> VISYDNYVTILDEETLKAWIAKLEKAPVFAFDTETDSLDNISANLVGLSFAIEPGVAAYIPVAHDYLDAPDQISRERALELLKPLLEDEKALKVGQNLKYDRGILANYGIELRGIAFDTMLESYILNSVAGRHDMDSLAERWLKHKTITFEEIAGKGKNQLTFNQIALEEAGRYAAEDADVTLQLHLKMWPDLQKHKGPLNVFENIEMPLVPVLSRIERNGVKIDPKVLHNHSEELTLRLAELEKKAHEIAGEEFNLSSTKQLQTILFEKQGIKPLKKTPGGAPSTSEEVLEELALDYPLPKVILEYRGLAKLKSTYTDKLPLMINPKTGRVHTSYHQAVTATGRLSSTDPNLQNIPVRNEEGRRIRQAFIAPEDYVIVSADYSQIELRIMAHLSRDKGLLTAFAEGKDIHRATAAEVFGLPLETVTSEQRRSAKAI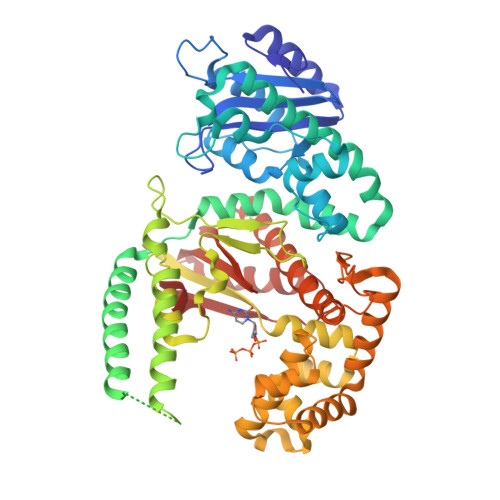NFGLIYGMSAFGLARQLNIPRKEAQKYMDLYFERYPGVLEYMERTRAQAKEQGYVETLDGRRLYLPDIKSSNGARRAAAERAAINAPMQGTAADIIKRAMIAVDAWLQAEQPRVRMIMQVHDELVFEVHKDDVDAVAKQIHQLMENCTRLDVPLLVEVGSGENWDQAH> MGMRRERDAEAELNLPPGFRFHPTDDELVEHYLCRKAAGQRLPVPIIAEVDLYKFDPWDLPE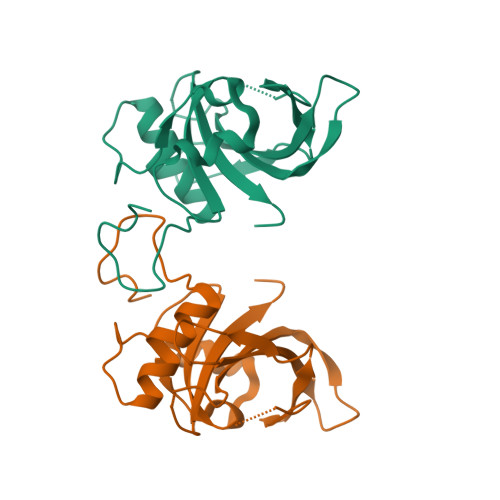RALFGAREWYFFTPRDRKYPNGSRPNRAAGNGYWKATGADKPVAPRGRTLGIKKALVFYAGKAPRGVKTDWIMHEYRLADAGRAAAGAKKGSLRLDDWVLCRLYNKKNEWEK>[2x]MKTLGEFIVEKQHEFSHATGELTALLSAIKLGAKIIHRDINKAGLVDILGASGAENVQGEVQQKLDLFANEKLKAALKARDIVAGIASEEEDEIVVFEGCEHAKYVVLMDPLD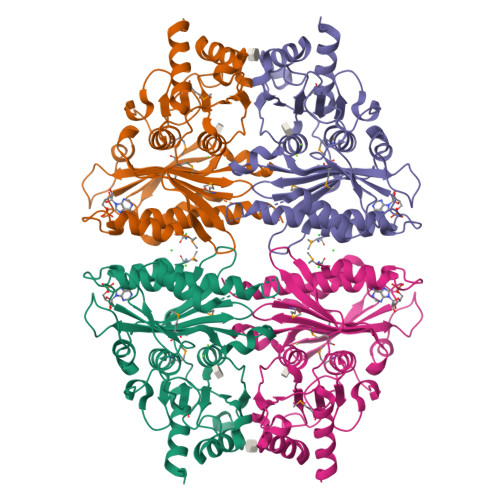GSSNIDVNVSVGTIFSIYRRVTPVGTPVTEEDFLQPGNKQVAAGYVVYGSSTMLVYTTGCGVHAFTYDPSLGVFCLCQERMRFPEKGKTYSINEGNYIKFPNGVKKYIKFCQEEDKSTNRPYTSRYIGSLVADFHRNLLKGGIYLYPSTASHPDGKLRLLYECNPMAFLAEQAGGKASDGKERILDIIPETLHQRRSFFVGNDHMVEDVERFIREFPDA>[2x]AALPQDEKLITGQLDNGLRYMIYPHAHPKDQVNLWLQIHTGSLQEEDNELGVAHFVEHMMFNGTKTWPGNKVIETFESMGLRFGRDVNAYTSYDETVYQVSLPTTQKQNLQQVMAIFSEWSNAATFEKLEVDAERGVITEEWRAHQDAKWRTSQARRPFLLANTRNLDREPIGLMDTVATVTPAQLRQFYQRWYQPNNMTFIVVGDIDSK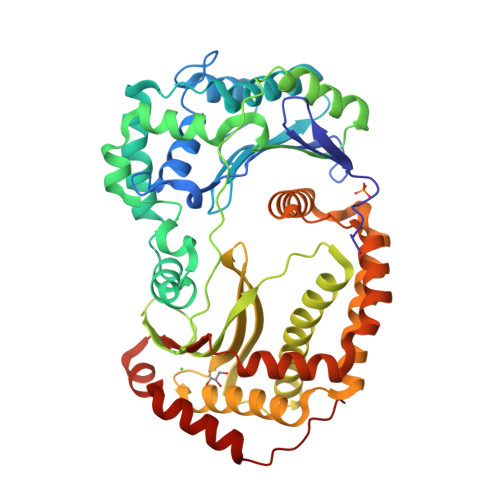EALALIKDNLSKLPANKAAENRVWPTKAENHLRFNIINDKENRVNGIALYYRLPMVQVNDEQSFIEQAEWSMLVQLFNQRLQERIQSGELKTISGGTARSVKIAPDYQSLFFRVNARDDNMQDAANALMAELATIDQHGFSAEELDDVKSTRLTWLKNAVDQQAERDLRMLTSRLASSSLNNTPFLSPEETYQLSKRLWQQITVQSLAEKWQQLRKNQDAFWEQMVNNEVAAKKALSPAAILALEKEYANKKLAAYVFPGR>MPIKVGINGFGRIGRMVFQALCEDGLLGTEIDVVAVVDMNTDAEYFAYQMRYDTVHGKFKYEVTTTKSSPSVAKDDTLVVNGHRILCVKAQRNPADLPWGKLGVEYVIESTGLFTAKAAAEGHLRGGARKVVISAPASGGAKTLVMGVNHHEYNPSEHHVVSNASCTTNCLAPIVHVLVKEGFGVQTGLMTTIHSYTATQKTVDGVSVKDWRGGRAAAVNIIPSTTGAAKAVGMVIPSTQGKLTGMSFRVPTPDVSVVDLTFTAARDTSIQEIDAALKRASKTYMKGILGYTDEELVSADFINDNRSSIYDSKATLQNNLPKERRFFKIVSWYDNEWGYSHR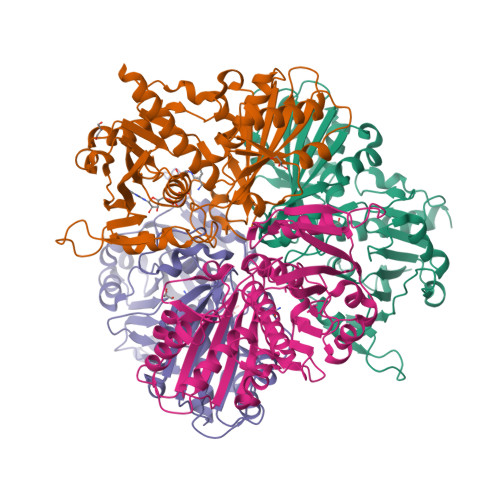VVDLVRHMASKDRSARL[4x]>[2x]SLFELGKMILQETGKNPAKSYGAYGCNCGVLGRGKPKDAT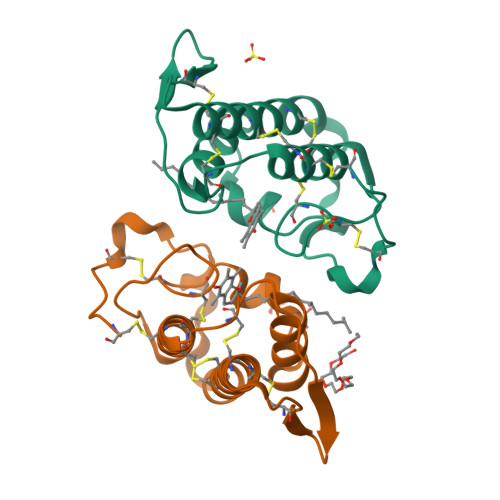DRCCYVHKCCYKKLTGCNPKKDRYSYSWKDKTIVCGENNPCLKELCECDKAVAICLRENLGTYNKKYRYHLKPFCKKADDC> MSSNRVLDLFKPFESFLPEVIAPERKVPYNQKLIWTGVSLLIFLILGQIPLYGIVSSETSDPLYWLRAMLASNRGTLLELGVSPIITSSMIFQFLQGTQLLQIRPESKQDRELFQIAQKVCAIILILGQALVVVMTGNYGAPSDLGLPICLLLIFQLMFASLIVMLLDELLSKGYGLGSGISLFTATNIAEQIFWRAFAPTTVNSGRGKEFEGAVIAFFHLLAVRKDKKRALVEAFYRTNLPNMFQVLMTVAIFLFVLYLQGFRYELPIRSTKVRGQIGIYPIKLFYTSNTPIMLQSALTSNIFLISQILFQKYPTNPLIRLIGVWGIRPGTQGPQMALSGLAYYIQPLMSLSEALLDPIKTIVYITFVLGSCAVFSKTWIEISGTSPRDIAKQFKDQGMVINGKRETSIYRELKKIIPTAAAFGGATIGALSVGSDLLGTLGSGASILMATTTIYGYYEAAAKEGGFTKNLVPGFSDLM;> MSSPTPPGGQRTLQKRKQGSSQKVAASAPKKNTNSNNSILKIYSDEATGLRVDPLVVLFLAVGFIFSVVALHVISKVAGKLF;> MARASEKGEEKKQSNNQVEKLVEAPVEFVREGTQFLAKCKKPDLKEYTKIVKAVGIGFIAVGIIGYAIKLIHIPIRYVIV;> GGSGGSGGSGGSGGSPTNYEYDEASETWPSFILTGLLMVVGPMTLLQIYQIFFGANAEDGNSGKSKEFNEEVFKNLNEEYTSDEIKQFRRKFDKNSNKKSKIWSRRNIIIIVGWILVAILLQRINSNDAIKDAATKLFDPYEILGISTSASDRDIKSAYRKLSVKFHPDKLAKGLTPDEKSVMEETYVQITKAYESLTDELVRQNYLKYGHPDGPQSTSHGIASGSGGSGGSASPLLVVCYVALLGLILPYFVSRWWARTQSYTKKGIHNVTASNFVSNLVNYKPSEIVTTDLILHWLSFAHEFKQFFPDLQPTDFEKLLQDHINRRDSGK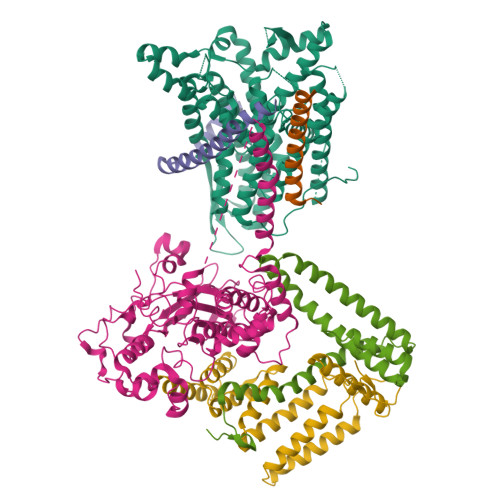LNNAKFRIVAKCHSLLHGLLDIACGFRNLDIALGAINTFKCIVQAVPLTPNCQILQLPNVDKEHFITKTGDIHTLGKLFTLEDAKIGEVLGIKDQAKLNETLRVASHIPNLKIIKADFLVPGRPYISLKVLVRSAKQPLIPTSLIPEENLTEPQDSESQRDPFAMMSKQPLVPYSFAPFFPTKRRGSWCCLVSSQKDGKILQTPIIIEKLSYKNLNDDKDFFDKRIKMDLTKHEKFDINDWEIGTIKIPLGQPAPETVGDFFFRVIVKSTDYFTTDLDITMNMKVRDSPAVEQVEVYSEEDDEYSTDDDETESDDESDASDYTDIDTDTEAEDDESPEGENLYFQ;> MSEFNETKFSNNGTFFETEEPIVETKSISVYTPLIYVFILVVSLVMFASSYRKKQAKKISEQPSIFDENDAHDLYFQIKEMSENEKIHEKVLKAALLNRGAESVRRSLKLKELAPQINLLYKNGSIGEDYWKRFETEVKLIELEFKDTLQEAERLQPGWVQLFVMVCKEICFNQALSRRYQSILKRKEVCIKEWELKINNDGRLVN;> MVTLEYNANSKLITASDAVVALSTETNIDQINVLTTSLIGETNPNFTPQPNEALSKMIKGLFESGMKNLQQKKLNEALKNVSLAIEMAQRKRAPWEAFAIQLPELHFMLRSKIDLCLILGKHLEALQDLDFLLGTGLIQPDVFVRKADCLLKLRQWEEARATCERGLALAPEDMKLRALLIETARNLAEYNGE>[2x]KWDYKNKENGPHRWDKLHKDFEVCKSGKSQSPINIEHYYHTQDKADLQFKYAASKPKAVFFTHHTLKASFEPTNHINYRGHDYVLDNVHFHAPME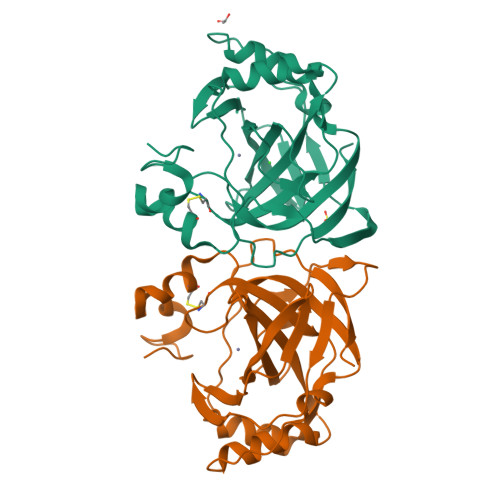FLINNKTRPLSAHFVHKDAKGRLLVLAIGFEEGKENPNLDPILEGIQKKQNFKEVALDAFLPKSINYYHFNGSLTAPPCTEGVAWFVVEEPLEVSAKQLAEIKKRMKNSPNQRPVQPDYNTVIIKRSAETR>MNPITSKFDKVLNASSEYGHVNHEPDSSKEQQRNTPQKSMPFSDQIGNYQRNKGIPVQSYDNSKIYIIGSGIAGMSAAYYFIRDGHVPAKNITFLEQLHIDGGSLDGAGNPTDGYIIRGGREMDMTYENLWDMFQDIPALEMPAPYSVLDEYRLINDNDSNYSKARLINNKGEIKDFSKFGLNKMDQLAIIRLLLKNKEELDDLTIEDYFSESFLKSNFWTFWRTMFAFENWHSLLELKLYMHRF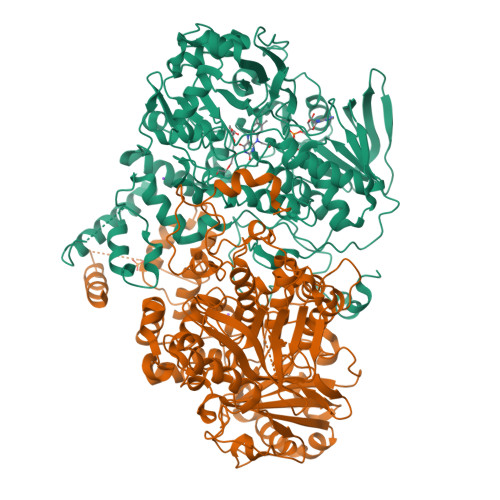LHAIDGLNDLSSLVFPKYNQYDTFVTPLRKFLQEKGVNIHLNTLVKDLDIHINTEGKVVEGIITEQDGKEVKIPVGKNDYVIVTTGSMTEDTFYGNNKTAPIIGIDNSTSGQSAGWKLWKNLAAKSEIFGKPEKFCSNIEKSAWESATLTCKPSALIDKLKEYSVNDPYSGKTVTGGIITITDSNWLMSFTCNRQPHFPEQPDDVLVLWVYALFMDKEGNYIKKTMLECTGDEILAELCYHLGIEDQLENVQKNTIVRTAFMPYITSMFMPRAKGDRPRVVPEGCKNLGLVGQFVETNNDVVFTMESSVRTARIAVYKLLNLNKQVPDINPLQYDIRHLLKAAKTLNDDKPFVGEGLLRKVLKGTYFEHVLPAGAAEEEEHESFIAEHVNKFREWVKGIRG[2x]> MKTEWPELVGKSVEEAKKVILQDKPEAQIIVLPVGTIVTMEYRIDRVRIFVDKLDNVAQVPRV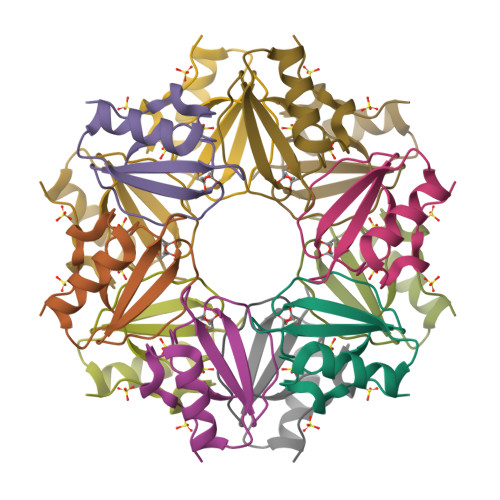G CISs are macromolecular injection devices with an overall structure that is homologous to the contractile tails of bacteriophages. Their conserved modules include an inner tube, a contractile sheath and a baseplate complex. For firing of the extended apparatus, the baseplate undergoes a conformational change and triggers sheath contraction, which in turn causes the inner tube to be expelled and injected into a target. Here we performed structural and mechanistic studies on a clade Ib CIS gene cluster in the marine bacterium Algoriphagus machipongonensis PR1.

All components of the tube initiator complex possess the conserved β-barrel folds seen in Alg1, whereas Alg7 has one additional C-terminal LysM domain extending out and interacting with the peripheral wedges. The central spike is surrounded by a hexagonal iris-like ring of Alg11-Alg12 heterodimers, forming the baseplate ‘wedges’ with the conserved core bundle and trifurcation units. Six copies of the gp25-like protein (Alg9) attach above Alg11-Alg12, where the C termini from two neighbouring protomers were observed to be slightly different. Like gp25 in the T4 phage, Alg9 mimics the ‘handshake’ to initiate sheath assembly and it interacts extensively with other baseplate components, implying a role in the initiation of contraction. Similar to Pvc12 and Afp12, Alg12 contains gp6-like and gp7-like parts. Domains I–III constitute the gp6-like part and participate in the assembly of the wedges, leaving the gp7-like part (domains IV–VII) exposed on the lateral surface of the baseplate. AlgoCIS exhibits a remarkable structural feature on the baseplate—the formation of an extensive ‘cage’ around the central spike. The Alg11 domain I forms the conserved core bundle together with the domains I and IV in Alg12. Interestingly, there is one additional large domain (IV, residues 278–643) protruding from the distal tip of domain III. The domains IV from the six protomers form a hexagonal cage that surrounds the spike (spike cage).

>[6x]MSTLNKHISIPKDMSSKDDLDFHFLREEGIRYIKELGSNFWTDYNTHDPGITMLEVLCYAISDLGNRINIPIEDLIANEEGGVKGQFYKVQEILPSAPTSELDLRKLFIDIEGIKNCWIKRERVTVFADLKNQKLSYEKTIWEDLKENQKAQFDLKGLYRILVETEDADKVLSESLEKAVFTKFHANRNLCEDLIKVEKVATEPISVCANVEVAPEADEELIHAQILIAIEDYLAPSPRHYSLKQMVDKGYTMDEIFEGPFLENGFIDTVELKASELRKEVRLSDIINIIMSIDGVKIVKEITLGNCDENDGIENNQWVICIPENKKPKLCKKTTINYFKGILPINLNPVRVDNHKSKILASRLENDLKAKDDLEPAIPQGTFADWGEYSSIQHEFPETYGISDIGLPPKLGVKRAVLARQLKGYLLFFDQILASYFEHLSKIKSLLSLDQGPSFTYFTQAIKDIKDVEELFKDPTLLENDEELTKSLIGKLDDTIERRNQLMDHLIARFAENFSSYAFLMKFLYGESTDEIVLQDKQSFLREYKEISRERGEGFNFYEQSNDNLWDTLNVSGAQKRISKLVGVKDYSRRNLSDTAVEIYRYEHVDGNWVYRWRIRDENGKVLLSATTSYPTYNSAGNEMYFAILKILETPLSDLEKLLEVNFRNENEAGSFHFHKAATSNKFSFDIINPVIDSESSSDFIVAKQYTYYPDRTQAVLGAISLLNFIKYTFTEEGIYLVEHILLRPSPLDPEYLAMQTDAGKEYIEGNFLPFCSDDYENCKMIDPYSFRVSIVLPGFTYRFANKDFRDYLENLIREELPAHIVAKICWIGYRKGEEPELFQEDVENPETPIFKENQLEIFEKAYKNYLFELTDIHKRKGFIASMNKYNQVLNEMTSSLTGLHTIYPTGRLYDCEDEEEELDGKLILGKTNLGTL;>MSENCNHIVTTLKRDGTGRRDLLDPKLAPESVQLQDFELSDWLIFALNFARKIHFFPSDLANEPLGDWRNFFSTIVSDKTLISDIENLDDFEKLRGNIEEFLAAYDQSGKLTPHLTLFVSFLKLLETSKKRFNQLTKRHLDFYYQEILHLEKQALSPDHVFLIFELAKNVSQEKLDEGTEVDGGKDDTGKKNTYLTSFETVLNKTKVGQLKSLYNEISVEKEEIKELNTPISTGTFVMAPMANSFDGLGEDFPKGSEKWWPFGYTKICNASTVLPALPKARLGCSISSKLLKLSEGTRDIILEFTFNKPILPNGEDYTALNKAMSIELTGEKGWIAGLPMTLKSDSGINSGSKKMKLSLTLDSEQPAVVPYQTELHEGSYEVDEPLLRVLFKTNEKEGYNLYRLFNENVLTDLKITVEVSDITSVQLENDLGVLNPQKPFFPFGPRPIKGSSFIVKYPEAMEKPVTAISYQMDYLNLPENLVNHYSAYTIGDDEPLVSDMDYFSVKSFPKSSNDSDQLFSEKSGGGYESDFEFQIENGVWESGLKKELKISLERSFLHEKYAHYFTLVAISKDTDPTIELLPNEPYAPLAENLVLGYTAISSIDFSSSSSENQVSLIHEMPFGFQQVFTPGDTDNSLYLVPDYCHGGELYIGLENGKNLQQVTLLLQFLEGSENPDITDIFTGNQKIKWQYLSQNQWQDFQSGEIIQNQTPRFLKSGIFQFSIPKQANLDNTVLPPGYHWIKASMVKPFDVVSQLINIHAQAVEAVFEDQGSSGNHLEKGLPAETISKLQERLSWIKSIQQPYPSTKGKAQESDEDYYRRVSERLRHKKRAITLWDYEHLILQKFPKVYKVKCLNHTCSSSFQSPGNATLILVPDTVQQSVFDIYQPRVSQGTLNDVAAFVNELNSFHVQAKVINPNYEEVKVDVKVKFREGLDVSFYLTKVKEDIKKFLSPWAYDQESSVEFGVTLHRSQMIHYLEQLTYVDYITDLRLLKRQAGSSPCNPIFIETTEKEYIQPSNPKSILVSAKEHLVTPITQNCSSISLNNEEECQH[6x];>MSEGKLEKLRIVAYKDSKFSDEVENGEFITLLNPEKYKFQYRVEQNEDQASGTSSAPIRFNKILPQTLEFDFLFDRTGVIAGYEVTEDGIINDIDHFKKVVYDYNGEKHKPNYLMITWGSLLFKGYLKEMDIEYKLFRPDGTPIRAMATTKIGEFVEEELRTAQENNQSPDMSHYRTVKEGDTLPLMTYRIYGDSKYYLEVAKANGLTNFRRLKTGTELIFPPLQKQK[6x];>[6x]MMEKSKDFLGTGWGFPPEFETSIGQVKTTSGVEDIQKSLEILFSTKIGERIMQPTYGCNLDELLFSPINRTLKTYVIELIKNAILYHEPRIDPEKIDITQGNEIEGELLIHLQYIVRATNSRKNMVYPFYLEEGTNI;>[6x]MATYYPPSSFHFLVEFTGIDAKNNDHEFQSVSGLSVDIDTEEFAEGGENRFKHKFPVKTKYPNLVLKRGVLVDSKVISWCRDAIEDFEFKPIDLTVKLLNEEHQPLMTWNVVHAYPVKWSVEDFNAQESKMAIESVELSYNYFKTIV;>MATYKTPGVYIEEITKFPPSVAQVETAIPAFIGYTQFARTKPSVDSDDLILKPKRISSLLDFTTYYGGAQNEQGITVKLTDTLIEGAENRTINVPEPTFKSPYLMFYSLQMYFANGGGPCYIVSTGVYDDWSDSETPPTINFSDLESGLAVIRKEDEPTLLLFPDATNLPTDDEFYSLYNSALMQCNDLQDRFTILDTYSDQTYNDGVEDLDPIPALRNGINLTKDYLKYGAAYYPFVQTILNYQYSADEIVIQHLSYNPNAIATALDNLNAVNGPTFIDAILDDLRDLSLPDISGEISDAVGFMYDDVDGFDIDGTFTTNSVKVANFASLVESVLSTLNELIDAKEEINKDVNSAIASSEEDNAIKTAISDALDVFNEDFEGADKIESVAKNLSDLLIKIKQADTNTKVENVLSINALNFSAEFEKLLTYDVNTGLTASVTLDLFANIGTRLDDIIAAVSAAEPIDVNNGKLNGRLLSDIEPLDNATYNTILLEINSHKVTLPPSSSMAGAYARVDNDRGVWKSPANIGLNYVSKPSVTVSHEEQESMNVHGTGKSVNAIRSFVGKGTLVWGARTLAGNDNEWRYISVRRFFNMAEESIKKATEQFVFEPNDGNTWVRVRAMIENFLILQWRAGALAGAKPEHAFYVKVGLGQTMTAQDILEGNMNVEIGLAVVRPAEFIILKFSHKMQES[6x];>MSYPLSKFHFSVEWGGTKIGFTEVSGLDLETEIIEYRHGASPEYSKIKMPGMQKFSNITLKRGTFKSDNEYFQWYNTINLNKVERRDLTISLLNEEHEPVVTWKVKNAWPLKVQSTDLKGDGNEVAIESMELAHEGLVIQNE[6x]>[4x]MEKTCADEFPLTVDSSEKQGVV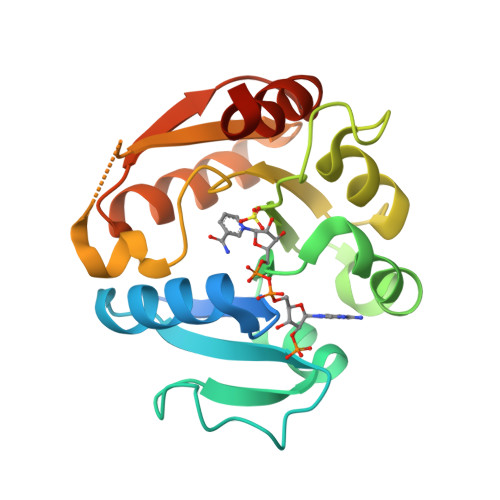CIFGTGDFGKSLGLKMLQCGYSVVFGSRNPQVSSLLPRGAEVLCYSEAASRSDVIVLAVHREHYDFLAELADSLKGRVLIDVSNNQKMNQYPESNAEYLAQLVPGAHVVKAFNTISAWALQSGTLDASRQVFVCGNDSKAKDRVMDIARTLGLTPLDQGSLVAAKEIENYPLQHHHHHH>MAEIGTGFPFDPHYVEVLGERMHYVDVGPRDGTPVLFLHGNPTSSYVWRNIIPHVAPTHRCIAPDLIGMGKSDKPDLGYFFDDHVRFMDAFIEALGLEEVVLVIHDWGSALGFHWAKRNPERVKGIAFMEFIRPIPTWDEWPEFARETFQAFRTTDVGRKLIIDQNVFIEGTLPMGVVRPLTEVEMDHYREPFLNPVDREPLWRFPNELPIAGEPANIVALVEEYMDWLHQSPVPKLLFWGTPGVLIPPAEAARLAKSLPNCKAVDIGPGLNLLQ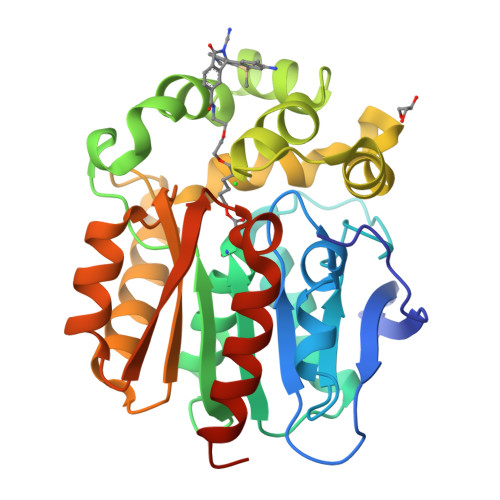EDNPDLIGSEIARWLSTLEISGHHHHHH[2x]> MKTETLYQDPVWFQDLSVIFKRPSEIIPTRDQSDSERINAMVRLVLYCSFAVALIRQNYL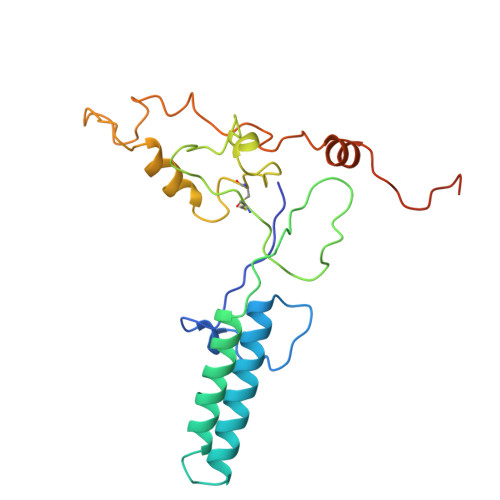YAILGLAIIAIISLAYALGAKKTKSNEAYGNIRPYSVKRSKKSCSKSSANNPFSNATVGALLDNEARPPACSYDDNDMASTMRKNFNKGLFRNLDDVYEVENSQRQFYTMPVTTAAPDLTAFGQFLYGSKGKTCKEDPSACTPAFATRDG> MARIHHHHHHGSDSIERRPVKDGGGTNSITVRNATFTWARSDPPTLNGITFSIPEGALVAVVGQVGCGKSSLLSALLAEMDKVEGHVAIKGSVAYVPQQAWIQNDSLRENILFGCQLEEPYYRSVIQACALLPDLEILPSGDRTEIGEKGVNLSGGQKQRVSLARAVYSNADIYLFDDPLSAVDAHVGKHIFENVIGPKGMLKNKTRILVTHSMSYLPQVDVIIVMSGGKISEMGSYQELLARDGAFAEFLRTYASTEQEQDAEE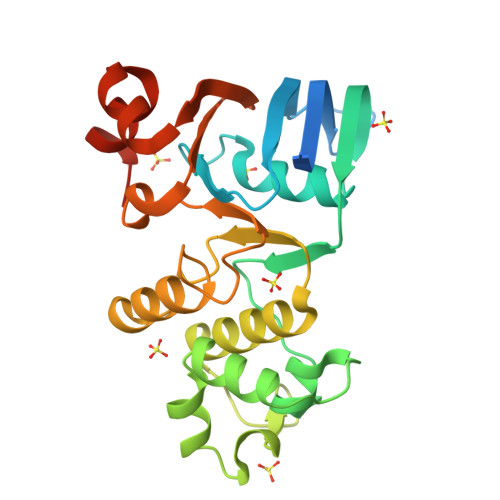N> MEHVAFGSEDIENTLAKMDDGQLDGLAFGAIQLDGDGNILQYNAAQGDITGRDPKQVIGKNFFKDVAPCTDSPEFYGKFKEGVASGNLNTMFEYT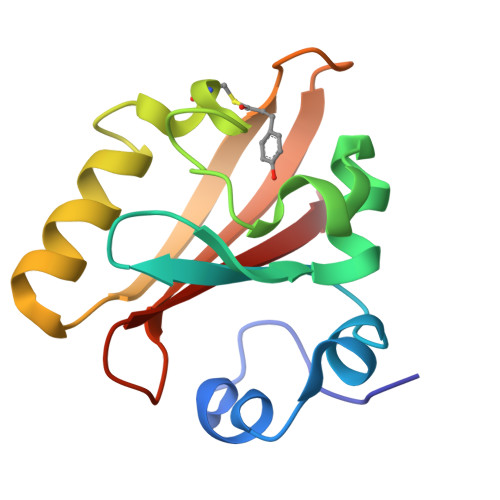FDYQMTPTKVKVHMKKALSGDSYWVFVKRV>MVCEGKRSASCPCFFLLTAKFYWILTMMQRTHSQEYAHSIRVDGDIILGGLFPVHAKGERGVPCGELKKEKGIHRLEAMLYAIDQINKDPDLLSNITLGVRILDTCSRDTYALEQSLTFVQALIEKDASDVKCANGDPPIFTKPDKISGVIGAAASSVSIMVANILRLFKIPQISYASTAPELSDNTRYDFFSRVVPPDSYQAQAMVDIVTALGWNYVSTLASEGNYGESGVEAFTQISREIGGVCIAQSQKIPREPRPGEFEKIIKRLLETPNARAVIMFANEDDIRRILEAAKKLNQSGHFLWIGSDSWGSKIAPVYQQEEIAEGAVTILPKRASIDGFDRYFRSRTLANNRRNVWFAEFWEENFGCKLGSHGKRNSHIKKCTGLERIARDSSYEQEGKVQFVIDAVYSMAYALHNMHKDLCPGYIGLCPRMSTIDGKELLGYIRAVNFNGSAGTPVTFNENGDAPGRYDIFQYQITNKSTEYKVIGHWTNQLHLKVEDMQWAHREHTHPASVCSLPCKPGERKKTVKGVPCCWHCERCEGYNYQVDELSCELCPLDQRPNMNRTGCQLIPIIKLEWHSPWAVV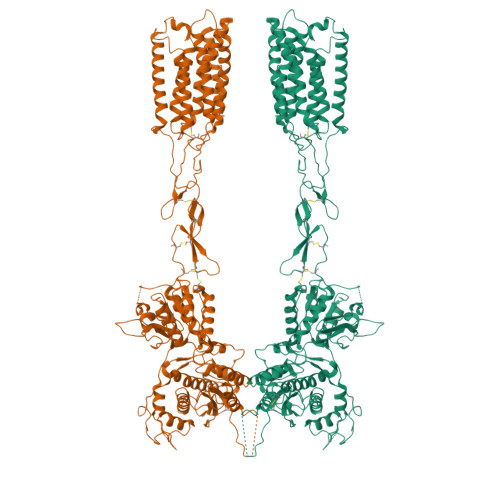PVFVAILGIIATTFVIVTFVRYNDTPIVRASGRELSYVLLTGIFLCYSITFLMIAAPDTIICSFRRVFLGLGMCFSYAALLTKTNRIHRIFEQGKKSVTAPKFISPASQLVITFSLISVQLLGVFVWFVVDPPHIIIDYGEQRTLDPEKARGVLKCDISDLSLICSLGYSILLMVTCTVYAIKTRGVPETFNEAKPIGFTMYTTCIIWLAFIPIFFGTAQSAEKMYIQTTTLTVSMSLSASVSLGMLYMPKVYIIIFHPEQNVQKRKRSFKAVVTAATMQSKLIQKGNDRPNGEVKSELCESLETNTSSTKTTYISYSNHSI[2x]> MKRILLSVLFIVFCLTAFVGCMKWDYGKMEPFRATGDGLFIMNEGNFQYGNATLSYYDPETKKVENEIFYRANAMKLGDVAQSMIVRDTIGWVVVNNSHVIFAISTNTFKEVGRITGLTSPRYIHFISDEKAYITQIWDYRIFIVNPKTYQITGYIECPDMTMETGSTEQMVQYGKYVYVNCWSYQNRILKIDTTTDKVVDQLTVGIQPTSLVMDKNFKM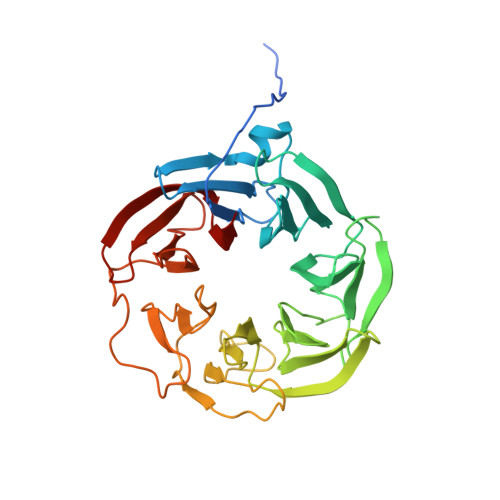WTITDGGYKGSPYGYEEPSLYRIDAETFKIEKQFKFQLGDAPSEVQLNGAGDELYWINKDIWRMSVDEERVPVRPFLKYRDTKYYGLTVSPKNGDVYVADAIDYQQQGMIYRYTEDGELVDEFYVGIIPGAFCWK>[4x]MKRVSRRAFLRRLGVGVAATAAFSPLAVAQARRYRWRIQTAWDAGTVGYSLFQKFTERVKELTDGQLEVQPFPAGAVVGTFDMFDAVKTGVLDGMNPFTLYWAGRMPVTAFLSSY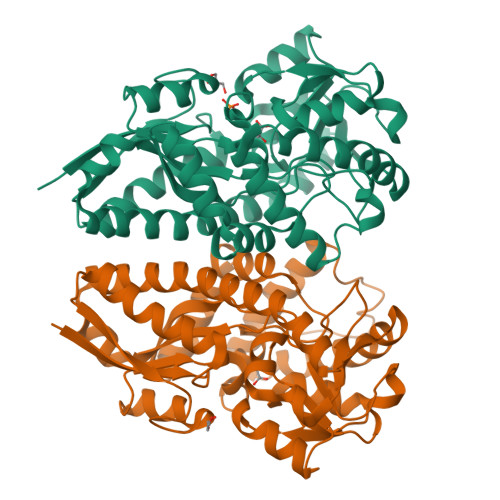ALGLDRPDQWETWFYSLGGLDIARRAFAEQGLFYVGPVQHDLNIIHSKKPIRRFEDFKGVKLRVPGGMIAEVFAAAGASTVLLPGGEVYPALERGVIDAADFVGPAVNYNLGFHQVAKYIIMGPPETPAIHQPVDLMDFTINLNRWRSLPKPLQERFIAAVHEYSWIHYAGIQKANLEAWPKYRQAGVEVIRLSNEDVRKFRRLAIPIWFKWAKMDKYSREAFASQLEYMKGIGYVTDEELKGLSL> GSHMTELTYTEEVVSIEKLKEDDEFKTLVPSNNSREDLEKSLREKSQIFPLIADRDYVLIDGYTRLDIMKKLGFKEVKILKYDFDSQQERDKAYELIWTFNGVRRQLNKNERLALFQKIADRIAKIQASKNKTEESKIVSHATQFSATESKQIEENEEFVTLDDGTTISALEYERILKELDKENKALSESDKRKMAILRINTPWLLKYVTDQKYKVPLDQAFRIYTRVKDLGILDKLKDLAPALRDPLITTREGRKIILNDEYRD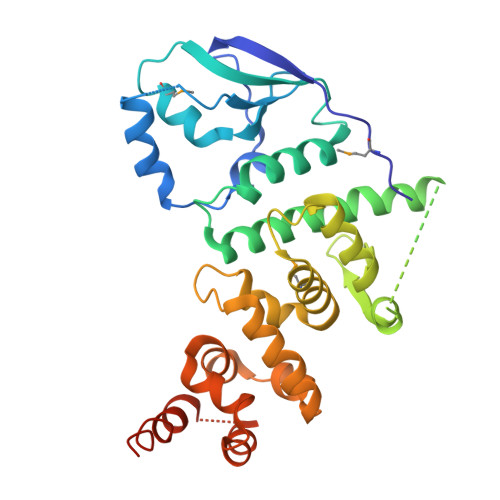LLEKIISKQYTTERAISVKQKEALKRGGKVKKSSK1-BROMOPROPANE-2-OL | C3 H7 Br O | 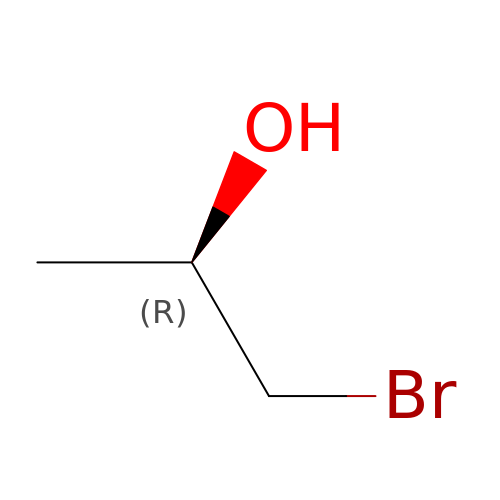WEGOLYBUWCMMMY-GSVOUGTGSA-N3-[(E,2S,4S)-2,4-dimethyloct-6-enoyl]-4-oxidanyl-1H-pyridin-2-one | C15 H21 N O3 | 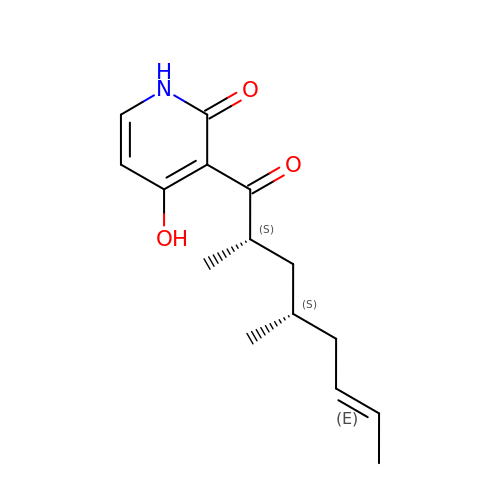XOAZFUVQLCZQIQ-NNOMMRTBSA-N> GGIQTSAAEATN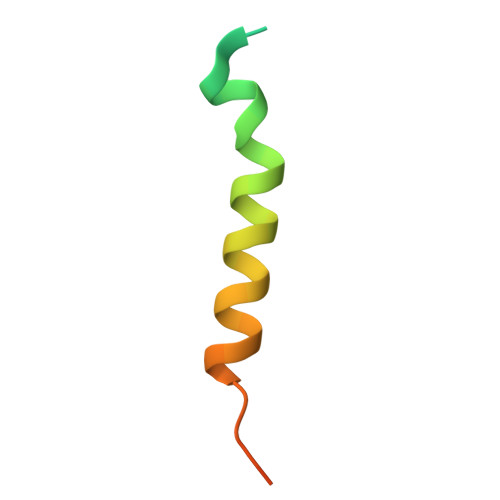STTSIVEMMQMPTQQLKQSVMDLLTYEGSNDMSGLS> MAVTDLSLTNSSLMPTLNPMIQQLALAIAASWQSLPLKPYQLPEDLGYVEGRLEGEKLVIENRCYQTPQFRKMELELAKVGKGLDILHCVMFPEPLYGLPLFGCDIVAGPGGVSAAIADLSPTQSDRQLPAAYQKSLAELGQPEFEQQRELPPWGEIFSEYCLFIRPSNVTEEERFVQRVVDFLQIHCHQSIVAEPLSEAQTLEHRQGQIHYCQQQQKNDKTRRVLEKAFGEAWAERYMSQV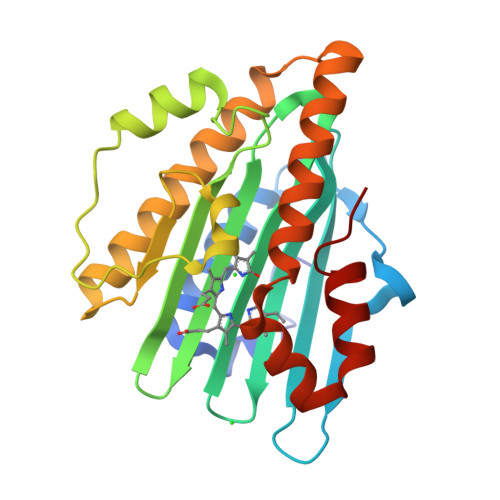LFDVIQ>[2x]SEFENPLKRLLVPGEEWEFEVTAFYRGRQVFQQTISCPEGLRLVGSEVGDRTLPGWPVTLPDPGMSLTDRGVMSYVRHVLSCLGGGLALWRAGQWLWAQRLGHCHTYWAVSEELLPNSGHGPDGEVPKDKEGGVFDLGPFIVDLITFTEGSGRSPRYALWFC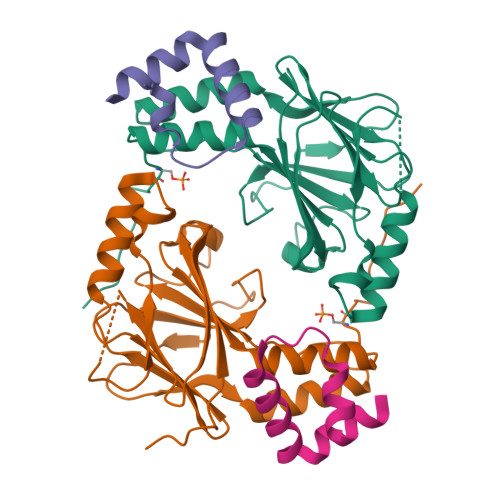VGESWPQDQPWTKRLVMVKVVPTCLRALVEMARVGGASSLENTVDLHISNS;>[2x]SALQDLLRTLKSPSSPQQQQQVLNILKSNPQLMAAFIKQRTAKYVAN> MSSERQ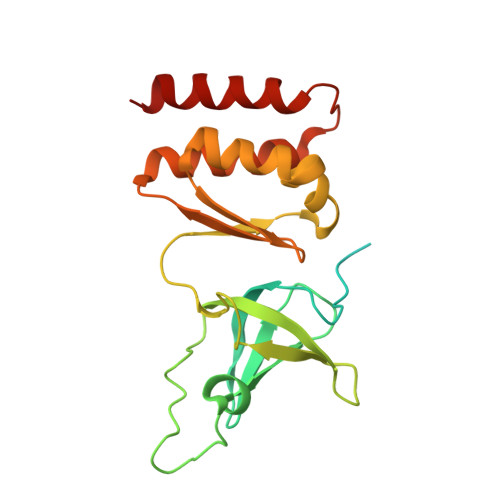LAGRIVVPGEPLPEEVEASPPYVIDYKGVKRATVVGLLREKGDGGGRAFVKLKEIYVPQAGDVVIGLIQSVGIMNWFVDINSPYVAVLSVQDFLGRPFNPAVDDMQSLLKVGDYIKAKVVAFDKTRSPLLTVQGEGLGRIVRGKIVEISPAKVPRVIGRKMSMLKTLEEKTECKIFVARNGRIHLECPNEDLEAIAVMAIKIIDEEAYTSGLTKRIIKFIEEERRIREV> GSHMASVYEPSLVDAYVGDDGAKKAVDGDLKTRVKFLGAPSTGDTIVYDLGQEILVDNLKYVVLDTEVDHVRDGKIQLSLDGETWTDAINIGDGVENGVDD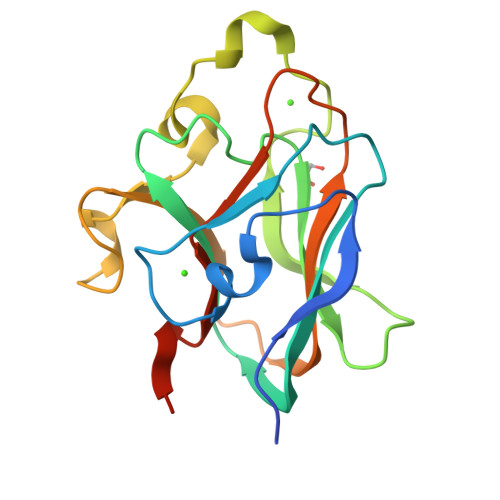MFSTPLKNGYKHGNQSGGIVPIDSAYVEGDNLNQKARYVRILFTAPYRHRWTVINELMINNGEYIPTVNDPT Here, a pipeline where crystals are grown in insect cells, sorted by flow cytometry and directly analysed by X-ray diffraction is presented and applied to in vivo-grown crystals of the recombinant CPV1 polyhedrin. In vivo crystallization has also been reported for the recombinant expression of heterologous polyhedrin proteins in insect cells, resulting in the formation of robust intracellular crystals of the cypovirus polyhedrin proteins that recapitulate their role in the infectious cycle as a crystalline armour around infectious particles. Of course, the CPV1 polyhedrin, like most examples of in vivo-grown crystals mentioned before, evolved to form crystals in the natural course of the infectious cycle. As reported in the first structure of the CPV1 polyhedrin, the ATP and CTP molecules have a very well defined electron density in the Fourier maps.

To compare in cellulo and purified crystals of the CPV1 polyhedrin, we compared these two types of crystals in parallel diffraction experiments. In cellulo and purified crystals had hit rates of 95.9% (two runs; n = 21 and n = 77) and 76.4% (two runs; n = 30 and n = 93), respectively. In contrast, omission of the cryoprotectant additive had no significant effect on in cellulo crystals. The best data sets for in cellulo (n = 9) and purified (n = 7) crystals were obtained by scaling the most isomorphous crystals using a total of nine and seven crystals, respectively. Based on a cutoff criterion of signal to noise decreasing to below 2.0 in the last resolution shell, the maximum resolution for each data set was 1.55 Å for the in cellulo data set and 1.90 Å for the purified crystal data set. p.i.m. is 7.5 and 17.3% for the two data sets processed at 1.90 Å resolution and collected from in cellulo and purified crystals, respectively. The refined occupancies are similar in both structures, suggesting that in this case the better map can be attributed to the higher resolution of the data rather than better ligand retention of the ligands in cells. By contrast, the average resolution of diffracting crystals is reproducibly superior for in cellulo crystals and the resolution limit of the best data set is improved by ∼0.35 Å compared with purified crystals. Importantly, the data collected in cellulo are of higher quality than the diffraction data obtained from purified crystals.

> XADVAGTSNRDFRGREQRLFNSEQYNYNNSLNGEVSVWVYAYYSDGSVLVINKNSQYKVGISETFKALKEYREGQHNDSYDEYEVNQSIYYPNGGDARKFHSNAKPRAIQIIFSPSVNVRTIKMAKGNAVSVPDEYLQRSHPWEATGIKYRKIKRDGEIVGYSHYFELPHEYNSISLAVSGVHKNPSSYNVGSAHNVMDVFQSCDLALRFCNRYWAELELVNHYISPNAYPYLDINNHSYGVALSNRQ5'-O-{(S)-hydroxy[(4-methyl-2-oxopentanoyl)oxy]phosphoryl}adenosine | 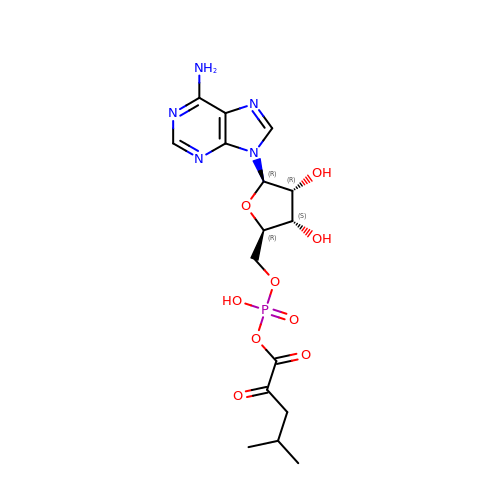C16 H22 N5 O9 P | QRKXCZFTEMACEI-SDBHATRESA-N((2-(6-amino-9H-purin-9-yl)ethyl)-L-seryl)phosphoramidic 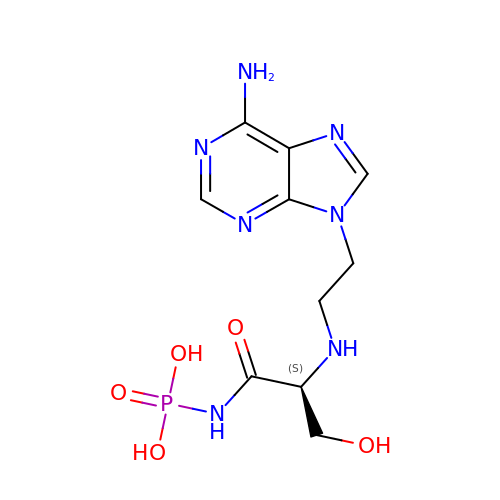acid | C10 H16 N7 O5 P | HTTMPVFKQATMIS-LURJTMIESA-N>GGIYGIGLDITELKRIASMAGRQKRFAERILTRSELDQYYELSEKRKNEFLAGRFAAKEAFSKAFGT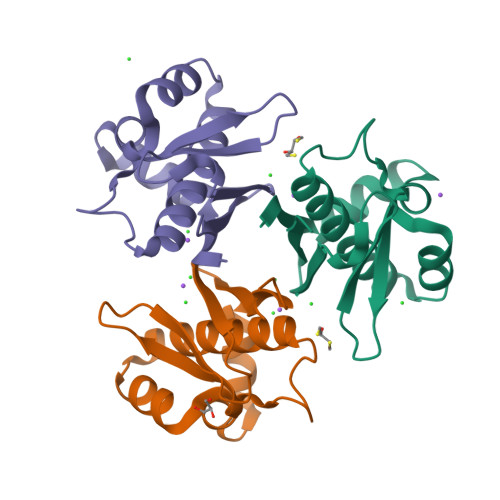GIGRQLSFQDIEIRKDQNGKPYIICTKLSPAAVHVSITHTKEYAAAQVVIERLSS[6x]> IGVCYGMLGNNLPPPSEVVSLYKSNNIARMRLYDPNQAALQALRNSNIQVLLDVPRSDVQSLASNPSAAGDWIRRNVVAYWPSVSFRYIAVGNELIPGSDLAQYILPAMRNIYNALSSAGLQNQIKVSTAVDTGVLGTSYPPSAGAFSSAAQAYLSPIVQFLASNGAPLLVNVYPYFSYTGNPGQISLPYALFTASGVVVQDGRFSYQNLFDAIVDAVFAALERVGGANVAVVVSESGWPSAGGGAEASTSNAQTYNQN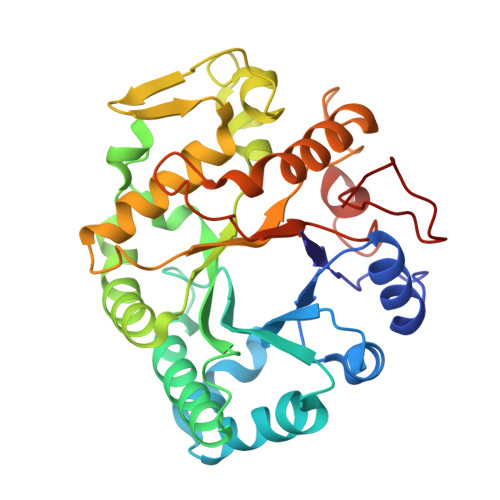LIRHVGGGTPRRPGKEIEAYIFEMFNENQKAGGIEQNFGLFYPNKQPVYQISF ethyl 4-[(4-chlorophenyl)amino]-4-oxidanylidene-butanoate | C12 H14 Cl N O3 | 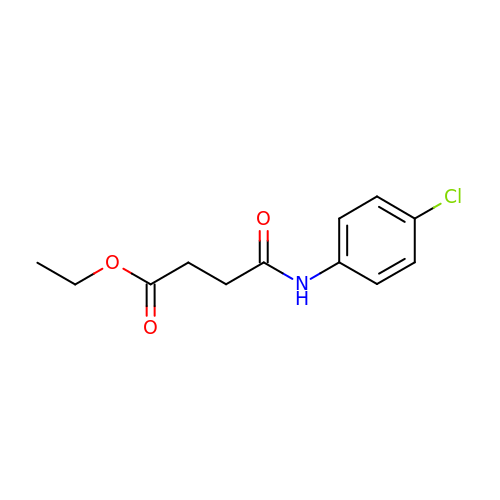XUFMMGCZRKBIFB-UHFFFAOYSA-N>[4x]GAMDPREVILCKDQDGKIGLRLKSIDNGIFVQLVQANSPASLVGLRFGDQVLQINGENCAGWSSDKAHKVLKQAFGEKITMTIRDRPFERTITMHKDSTGHVGFI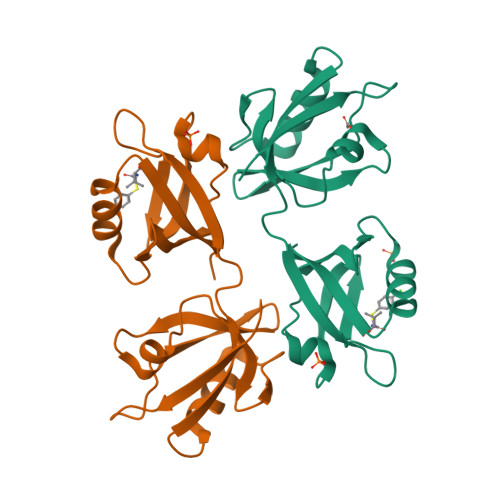FKNGKITSIVKDSSAARNGLLTEHNICEINGQNVIGLKDSQIADILSTSGTVVTITIMPAF> MGLISDPVEVDPIQVGRD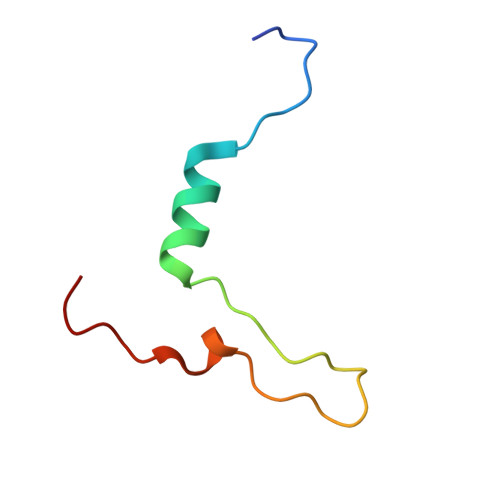EAGWVQELRDREAWPKQEVPEQAKKPAKVGN The present study focuses on the ancestor SMS from the hyperthermophilic archaeon Methanocaldococcus jannaschii. Biochemical and structural studies showed that SMS is made of a SmsC2B2 heterotetratmer wherein the SmsC subunit hosts both ATP and [Fe-S] cluster binding sites. With respect to the six components of the SUF system, SMS has only two components, SmsC and SmsB, encoded by the smsCB operon. The SmsC subunit, consisting of a RecA-like domain and a helical domain, contains all the structural motifs of the nucleotide-binding (NBD) subunits of the ABC ATPases (i.e., Walker A, Walker B, ABC signature, D-, Q-, and H-loops).

We set up crystallization conditions both under oxic and anoxic conditions and we obtained crystals of SmsC2B2 in both conditions. To obtain a nucleotide-bound structure, the crystals of SmsC2B2 grown in oxic conditions were soaked with 10 mM adenosine-5′-[(β,γ)-imido]triphosphate (AMP-PNP). SmsB and SmsC assembled into a symmetric hetero-tetramer consisting of two subunits of each protein related by a 2-fold symmetry. The SmsB subunits consist of a right-handed β-helix core domain (residues 33–289) connected by a short linker to a helical hairpin that serves as an anchoring point for SmsC, analogous to the coupling helices of the transmembrane subunits of ABC transporters. The first N-terminal 32 residues of SmsB are disordered and were not included in the final model. The two SmsB subunits tightly interact through an extended dimeric interface, which together with the two SmsB-SmsC contact interfaces stabilizes the hetero-tetrameric assembly. Most of the interactions between SmsC and the nucleotide are similar to those observed in other NBD structures of ABC transporters. (b) Close-up on the binding site of the AMP-PNP/Mg2+ showing residues surrounding the binding site of AMP-PNP.

> GEFMVSIMLLKVEDLHVYRGNREILKGVNLTVEENEIHAIIGPNGAGKSTLAYTIMGISGYKPTKGRIIFKGVDIIDKNITERARMGMTLAWQEPARFEGIKVKNYLMLGMNEKYKKDKEIAEEKIREALKLVNLDPDKYLDRYVDETLSGGERKRIELASIICMEPDLAILDEPDSGIDIVSFDEIKRVFDYLKDKGCSLLVITHREELAEHADRVSLICAGEVIKSGDPKEVGEFYKKECGKCYKKVPDGK;> MSIKEELMEIIEAIKYTSEKPEEIVHGKGPRIIVKESRIIDVQGDEGIILEGKEEDGKIKAKIIVKKGYKFKYPIHMCFGITEENISQIIDVEIILEEDSSISLMSHCSFPKGKGIKHIMNGIIKIGKNAKFSYNEFHYHGMDGDILVKPTVKVEIDEGGIYISNFTLTKGRIGTLDIEQEIIAKKDAIIDITTRTYAIKEDVVKVNEVVKLNGENAKCIIKSRGAAMDNSKISLKLKIEGNAPYSKGHIDCAEIVKGNAEVESIPIVVVRDDKARITHEAAIGSVDKKQLETLMAKGLDEDEATEIIVKGMIGDL> MWFGEFGGQ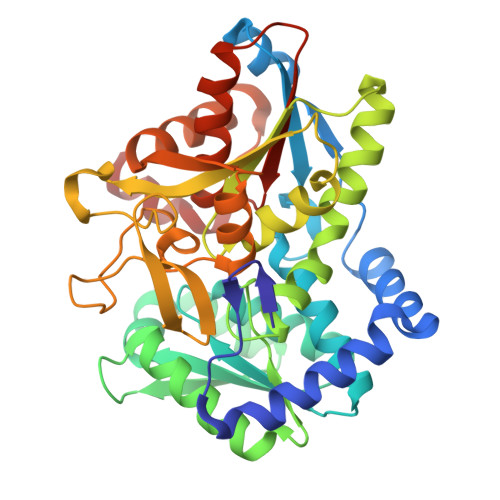YVPETLIEPLKELEKAYKRFKDDEEFNRQLNYYLKTWAGRPTPLYYAKRLTEKIGGAKIYLKREDLVHGGAHKTNNAIGQALLAKFMGKTRLIAETGAGQHGVATAMAGALLGMKVDIYMGAEDVERQKMNVFRMKLLGANVIPVNSGSRTLKDAINEALRDWVATFEYTHYLIGSVVGPHPYPTIVRDFQSVIGREAKAQILEAEGQLPDVIVACVGGGSNAMGIFYPFVNDKKVKLVGVEAGGKGLESGKHSASLNAGQVGVFHGMLSYFLQDEEGQIKPTHSIAPGLDYPGVGPEHAYLKKIQRAEYVTVTDEEALKAFHELSRTEGIIPALESAHAVAYAMKLAKEMSRDEIIIVNLSGRGDKDLDIVLKVS> MRIIKPFAILTPQTIIQDKAVAFDKKIEAIDTVENLIKKYPNAAVEHDENSLLLPGFANPHLHLEFSANKATLQYGDFIPWLYSVIRHREDLLPLCDGACLEQTLSSIIQTGTTAIGAISSYGEDLQACIDSALKVVYFNEVIGANAATADVMYASFLERFHQSKKHENERFKAAVAIHSPYSVHYILAKRALDIAKKYGSLVSVHFMESRAEREWLDKGSGEFAKFFKEFLNQTRPVNDTKSFLELFKELHTLFVHMVWANEEEIQTIASYNAHIIHCPISNRLLGNGVLDLEKIKSIPYAIATDGLSSNYSLNMYEELKAALFVHPNKEATTFAKELIIRATKAGYDALGFEGGEIAV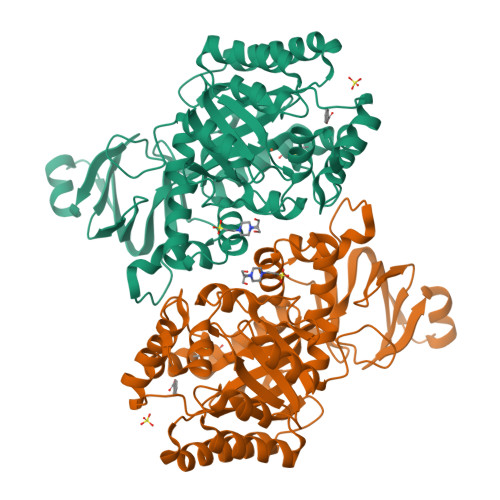GKDADMQLIDLPEGLTNVEDLYLHVILHTTKPKKVYIQGEEHVREAENLYFQSHHHHHHWSHPQFEK>GSELTLRTIADEDDYESYMASAYSVFLRDPQKDEIEVNRKFTELDRMIGFHDGKKWVATTGAFSRHVVLPGGAVVPVAAVTAVTVSPTHRRRGLLTTMMRHQLADIRSRGESLAMLFASEALIYGRFGYGVATESAELSGQVRELAFRPTVDLGDGTLEEVSAETFLASAPAIYDAVIPGLPGQMSRTPEWWASWTLDSEELQKESGKVRFVLHYESDGTASGFAIYRPKPGWGDAGPNAELHVQEVLGTNPRSYARTWRYLLDMDLVRKIKYHGASVQEELRYLVA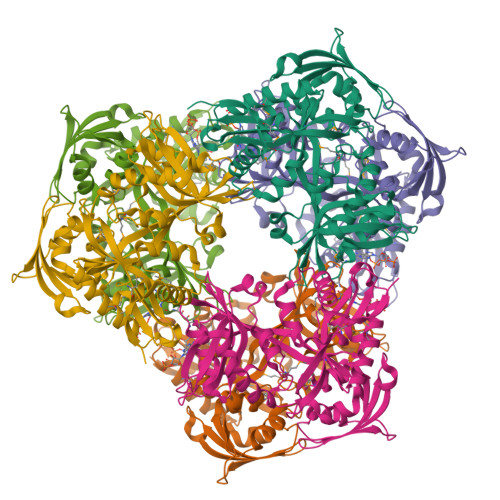NHPSLECVVSDAIQVRLVDIPRALAQRRYAADVDVVLEVTDDFLPENSGRYRLRGGLDHASCEITTDDADIALTVRDLGSVYMGGVSLQVLASAGLVTELRAGAVQRAATAFGWPVAPSAPDDF[6x]> FQTQKPLKSTSLSLFYKKVYRLAYLRLNTLCERLLSEHPELEHIIWTLFQHTLQNEYELMRDRHLDQIMMCSMYGICKVKNIDLKFKIIVTAYKDLPHAVQETFKRVLIKEEEYDSIIVFYNSVFMQRLKTNILQYASTRP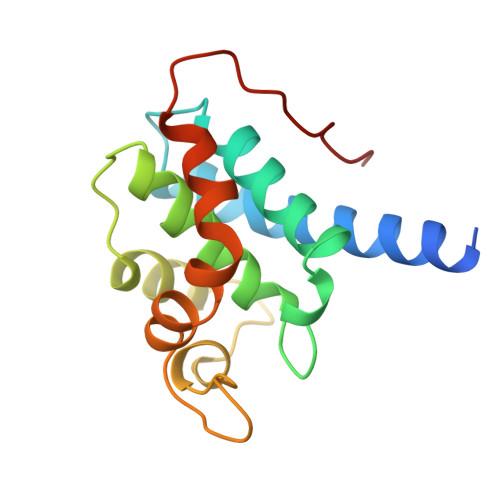PTLSPIPHIPR> SAAQKFVKQVIREAFLQDASDIHIEPRQNDVQVRLRIDGALRPYS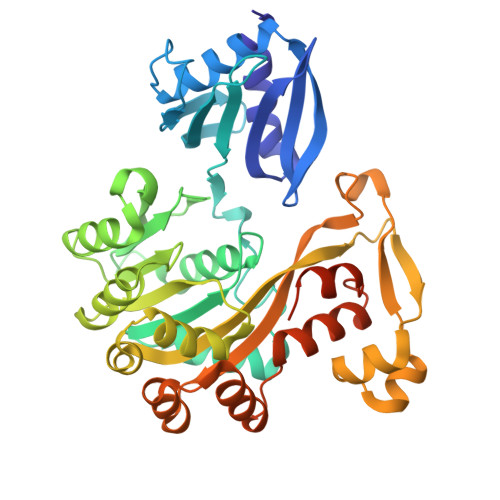TLPKGALNAVISVVKIMGGLNIAEKRLPQDGRVRYREGAIDVDLRLSTLPTVYGEKAVMRLLKKASDIPEIEDLGFAPGVFERFKEVISKPYGIFLITGPTGSGKSFTTFSILKRIATPDKNTQTIEDPVEYEIPGINQTQVNPQAGLTFARALRAFLRQDPDIIMVGEIRDSETAKIATEAALTGHLVIATLHTNDAAQAITRLDEMGVEPFNISAALIGVLSQRLVRRVCEHCKVEVKPDPETLRRLGLSEAEIQGARLYKGMGCERCGGTGYKGRYAIHELLVVDDEIRHAIVAGKSATEIKEIARRKGMKTLREDGLYKALQGITTLEEVLARTIEAAAELALVPRGSSAHHHHHHHHHH>[2x]GGYAGAS

Although other intermediate filament proteins have been demonstrated to form amyloids, KRT8 specifically has not previously been characterized as an amyloid-forming protein. This protein, like other alpha-keratin proteins, contains a central coiled-coil domain that is flanked by an amino-terminal head domain and a carboxy-terminal tail domain, which are both low complexity in sequence composition. KRT8 is known to aggregate pathologically, primarily in the form of MDBs in liver disease. Atomic structures of KRT8 LARKS reveal that pathogenic mutations convert the non-pleated wild-type protein into a pleated conformation, shedding light on the molecular mechanisms underlying aggregation-promoting mutations in low-complexity proteins.

Similarly, the structure of KRT852–58 (GGYAGAS) with the G55A mutation was also determined. High-resolution diffraction data were collected for the wild-type sequence (GGYGGAS) of KRT852–58, but we were unable to determine the structure, presumably owing to its adoption of a highly kinked conformation. Fortunately, a recently determined structure from hnRNPA1 (GGGYGGS) very closely resembles the wild-type KRT852–58 sequence, particularly the residues at and surrounding the mutation site, providing the needed comparison. The KRT852–58-G55A (GGYAGAS) structure forms an anti-parallel class-6 steric zipper, with sheets interacting through the tyrosine and two alanine residues, including the G55A mutant alanine. The glycine at the N terminus assumes a highly extended conformation, like the SGMGGIT structure. But, like the other mutant structure, the backbone at the mutant alanine is pleated. Comparison with GGGYGGS from hnRNPA1, which has the same GGYGG sequence motif as wild-type KRT852–58 (GGYGGAS), reveals that a glycine at that position adopts a highly extended backbone conformation. Similar to G62C, backbone overlay with the G55A mutation converts a non-pleated Gly55 into a pleated Ala55 (right). An overlay of both wild-type–mutant structure pairs highlights that mutations from wild-type glycines facilitate a transition in the backbone from a non-ideal, highly extended conformation to a pleated one. From these fibril structures, we observe that both the G62C and G55A mutations in KRT8 convert a non-pleated beta-sheet into a pleated one, transitioning a LARKS-like conformation into a steric zipper.>GPLGSFGQTTPPLVDFLKDILRRYPEGGQILKELIQNAEDAGATEVKFLYDETQYGTETLWSKDMAPYQGPALYVYNNAVFTPEDWHGIQEIARSRKKDDPLKVGRFGIGFNSVYHITDVPCIFSGDQIGMLDPHQTLFGPHESGQCWNLKDDSKEISEL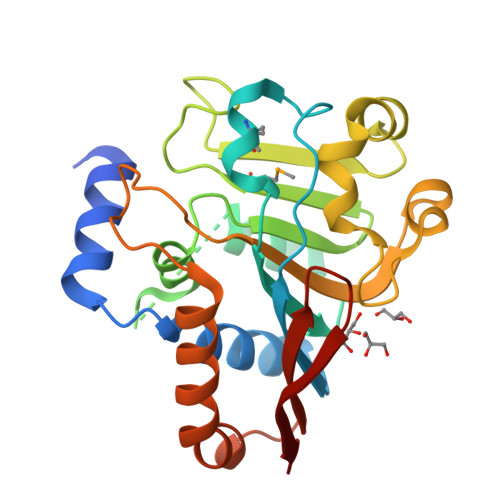SDQFAPFVGIFGSTKETFINGNFPGTFFRFPLRLQPSQLSSNLYNKQKVLELFESFRADADTVLLFLKSVQDVSLYVREADGTEKLVFRVTSS[3x]>[2x]MIAAQLLAYYFTELKDDQVKKID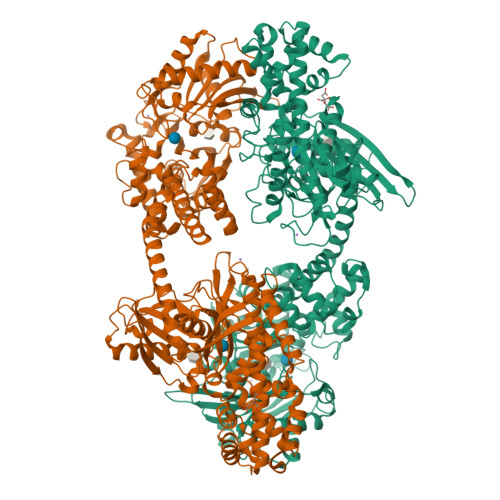KYLYAMRLSDETLIDIMTRFRKEMKNGLSRDFNPTATVKMLPTFVRSIPDGSEKGDFIALDLGGSSFRILRVQVNHEKNQNVHMESEVYDTPENIVHGSGSQLFDHVAECLGDFMEKRKIKDKKLPVGFTFSFPCQQSKIDEAILITWTKRFKASGVEGADVVKLLNKAIKKRGDYDANIVAVVNDTVGTMMTCGYDDQHCEVGLIIGTGTNACYMEELRHIDLVEGDEGRMCINTEWGAFGDDGSLEDIRTEFDREIDRGSLNPGKQLFEKMVSGMYLGELVRLILVKMAKEGLLFEGRITPELLTRGKFNTSDVSAIEKNKEGLHNAKEILTRLGVEPSDDDCVSVQHVCTIVSFRSANLVAATLGAILNRLRDNKGTPRLRTTVGVDGSLYKTHPQYSRRFHKTLRRLVPDSDVRFLLSESGSGKGAAMVTAVAYRLAEQHRQIEETLAHFHLTKDMLLEVKKRMRAEMELGLRKQTHNNAVVKMLPSFVRRTPDGTENGDFLALDLGGTNFRVLLVKIRSGKKRTVEMHNKIYAIPIEIMQGTGEELFDHIVSCISDFLDYMGIKGPRMPLGFTFSFPCQQTSLDAGILITWTKGFKATDCVGHDVVTLLRDAIKRREEFDLDVVAVVNDTVGTMMTCAYEEPTCEVGLIVGTGSNACYMEEMKNVEMVEGDQGQMCINMEWGAFGDNGCLDDIRTHYDRLVDEYSLNAGKQRYEKMISGMYLGEIVRNILIDFTKKGFLFRGQISETLKTRGIFETKFLSQIESDRLALLQVRAILQQLGLNSTCDDSILVKTVCGVVSRRAAQLCGAGMAAVVDKIRENRGLDRLNVTVGVDGTLYKLHPHFSRIMHQTVKELSPKCNVSFLLSEDGSGKGAALITAVGVRLRTEASS(2R)-N~2~-(3-chloro-4-cyanophenyl)-N~4~-[3-(cyclopropylmethyl)-2,4-dioxo-1-(propan-2-yl)-1,2,3,4-tetrahydroquinazolin-6-yl]morpholine-2,4-dicarboxamide 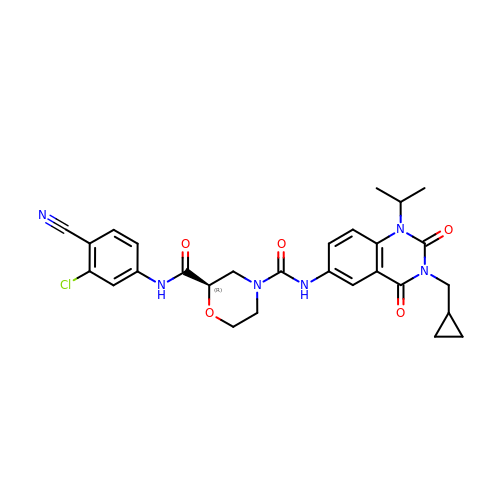| C28 H29 Cl N6 O5 | QUTSLTZISBFEOJ-XMMPIXPASA-N> RPP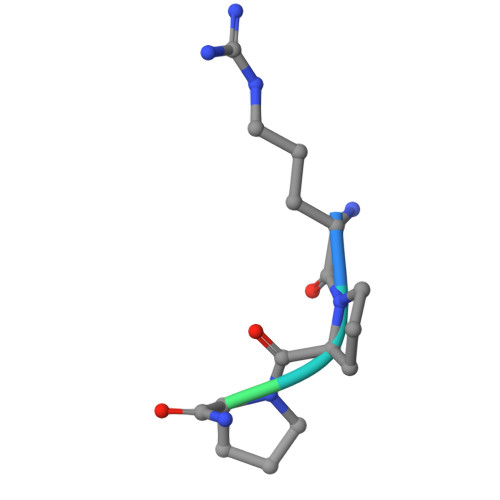GFTPFR> TFISRFAPDQPRKGADILVEALERQGVETVFAYPGGASMEIHQALTRSSSIRNVLPRHEQGGVFAAEGYARSSGKPGICIATSGPGATNLVSGLADALLDSVPLVAITGQVTRRMIGTDAFQETPIVEVTRSITKHNYLVMDVEDIPRIIEEAFFLATSGRPGPVLVDVPKDIQQQLAIPNWEQAMRLPGYMSRMPKPPEDSHLEQIVRLISESKKPVLYVGGGCLNSSDELGRFVELTGIPVASTLMGLGSYPCDDELSLHMLGMHGTVYANYAVEHSDLLLAFGVRFDDRVT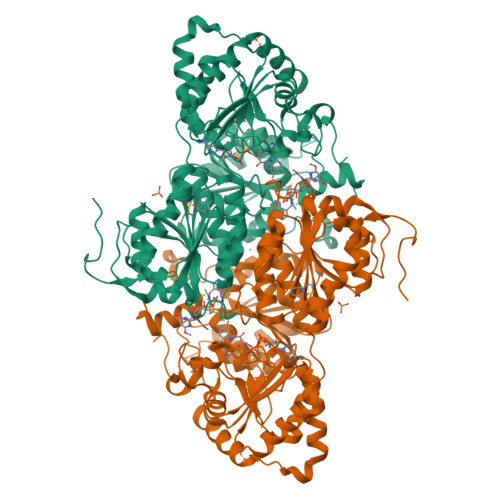GKLEAFASRAKIVHIDIDSAEIGKNKTPHVSVCGDVKLALQGMNKVLENRAEELKLDFGVWRNELNVQKQKFPLSFKTFGEAIPPQYAIKVLDELTDGKAIISTGVGQHQMWAAQFYNYKKPRQWLSSGGLGAMGFGLPAAIGASVANPDAIVVDIDGDGSFIMNVQELATIRVENLPVKVLLLNNQHLGMVMQWEDRFYKANRAHTFLGDPAQEDEIFPNMLLFAAACGIPAARVTKKADLREAIQTMLDTPGPYLLDVICPHQEHVLPMIPSGGTFNDVITEGDGR> VFHKIRNEDLIFNESLGQGTFTKIFKGVRREVGDYGQLHETEVLLKVLDKAHRNYSESFFEAASMMSKLSHKHLVLNYGVCFCGDENILVQEFVKFGSLDTYLKKNKNCINILWKLEVAKQLAWAMHFLEENTLIHGNVCAKNILLIREEDRKTGNPPFIKLSDPGISITVLPKDILQERIPWVPPECIENPKNLNLATDKWSFGTTLWEICSGGDKPLSALDSQRKLQFYEDRHQLPAPKAAELANLINNCMDYEPDHRPSFRAIIRDLNSLFTPDLVPRGSHHHHHH

JAK2, like other JAK family members, comprises a catalytically active C-terminal tyrosine kinase domain (JH1), a regulatory pseudokinase domain (JH2), and a Src homology-2 (SH2)-like domain that, together with the N-terminal FERM (N-terminal 4.1, ezrin, radixin, moesin) domain, forms the major receptor interaction moiety. The JH2 domain has a key role in mediating both negative and positive regulation of JAK kinase activity and numerous disease mutations locate in JH2, including the prevalent hyperactivating JAK2 V617F in MPN. Previous studies have demonstrated that JAK2 JH2 binds ATP and possesses regulatory autophosphorylation activity on Ser523 and Tyr570. To gain insights on the compound binding modes to JAK2 JH2 and to analyze whether any differences could be observed between binding to WT and V617F, we determined the crystal structures of selected small molecules with JAK2 JH2 WT and V617F.

The TSA screens identified six compounds that induced shift in the unfolding temperature of recombinant JAK2 JH2 V617F at or above 2 °C, four of which were identified from collection screened only by TSA and two, JNJ-7706621 (1) and AT9283 (2), from collections screened by TSA and FP. JNJ-7706621 (1) and AT-9283 (2) were also observed as JAK2 JH2 binders in a previous screening by Puleo and coworkers. The initial hits 1 and 2 possessed highly JH1-selective binding over JH2 on JAK2, whereas JH1-selectivity of 7 was minor. Compounds 1, 2, and 7 also inhibited viability of MPN model cell lines HEL and SET-2, both of which express JAK2 V617F (homozygous in HEL, heterozygous in SET-2), and murine pro-B cells Ba/F3 carrying either hJAK2 wildtype or V617F at submicromolar-micromolar range. Structural analysis of compound binding modes to JAK2 JH2 WT and V617F mutant revealed no major differences in the binding modes with the exception of compound 1. 1 interacts with the side chain of Ser698 in the WT structure but in V617F structure this serine assumes two conformations and instead of interacting with the serine, 1 forms a hydrogen bond with Lys581, which is shifted closer to the compound. In addition, 1 forms an H-bond with the side chain of Lys640 from the αD helix. This interaction is also not present in the WT structure. Differences observed in the complexes with 1 stem from the conformation of the Gln626, the αD lysine and differences at the back of the binding pocket. The variation in the hydrogen bonding pattern in the back of the pocket (Ser698 in WT vs. Lys581 in V617F) might reflect differences in the dynamics of the pocket between the structures but altogether the differences in hydrogen bonding with 1 is not reflected on IC50 values.> MLNTQTIIDVNKAMDAMLRAYLNQDIAIRFDLPELDTMQSDAMVSIFLYDIHEDLQLRSAESRGFDVYAGRLLPGWVNIKCNYLITYWEASKPATDASSPDSQPDNQAIQVMSQVLNALINNRQLAGIPGAYTQVVPPKESLNSLGNFWQSLGNRPRLSLNYSVTVPVSLNDGQDSATPVTAVSSTVEQTASLSQEVVSHALRELLITELGGGEDNRLVLSKVELSAVKETMTQDSPAQMIILLSVSGITRQEYLKEIDNIFDRWVNNAEVITTIDDCGIRIESITKDNLVG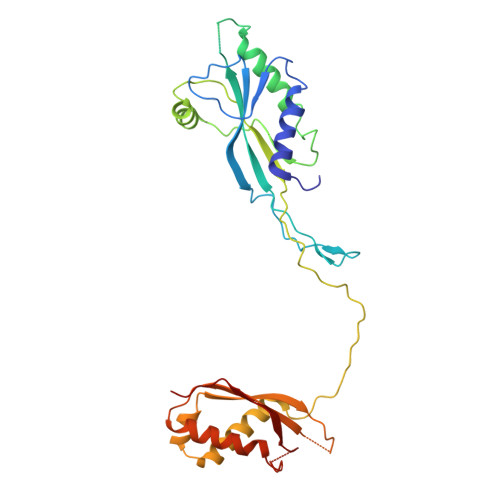I> IVGGQECKDGECPWQALLINEENEGFCGGTILSEFYILTAAHCLYQAKRFKVRVGDRNTEQEEGGEAVHEVEVVIKHNRFTKETYDFDIA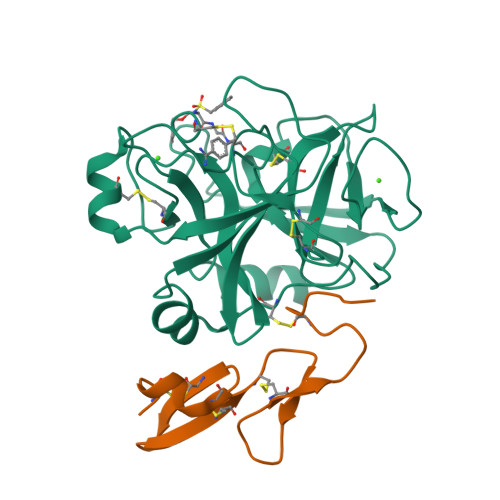VLRLKTPITFRMNVAPACLPERDWAESTLMTQKTGIVSGFGRTHEKGRQSTRLKMLEVPYVDRNSCKLSSSFIITQNMFCAGYDTKQEDACQGDSGGPHVTRFKDTYFVTGIVSWGEGCARKGKYGIYTKVTAFLKWIDRSMKT;> LCSLDNGDCDQFCHEEQNSVVCSCARGYTLADNGKACIPTGPYPCGKQTLE> GHMSFKNFKVVEKMIFGRGSFVQLDDVLAAQRKADDDFVVFLVDDVHQGKPLEARIPVKAQDL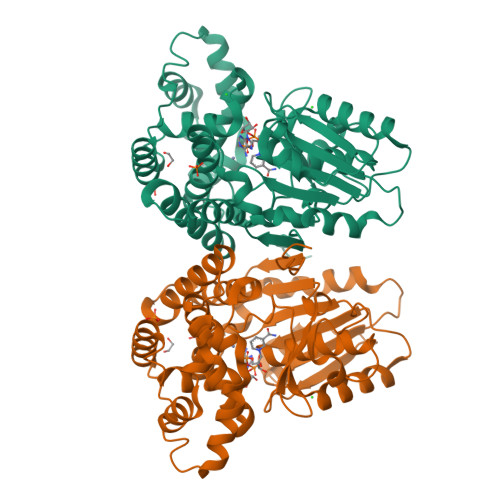LIWVNVDEEPSTIQIDALTEQVQAFNGKLPVSVVGLGGGSTMDVAKAVSLMLTNPGGSAMYQGWDLIKKPAVHHIGIPTISGTGAEASRTAVLCGPVRKLGLNSDYTVFDQIIMDSELIDGVETDQWFYTGMDCYIHCVESLEGTFLNEFSKAYAEKAMDLCRQVYLEDHPEKDDKLMMASFMGGMSIAYSQVGACHAVSYGLSYILGYHHGIGNCIAFDVLEEFYPEGVAEFRLMMKKHNITLPKNICKDLPDETIAKMVAVTKSMGPLWANVYGPTWEEKVTDEMLTALFRRI>[3x]SLSPAVQTFWKWLQEEGVITAKTPVKASVVTEGLGLVALKDISRNDVILQVPKRLWINPDAVAASEIGRVCSELKPWLSVILFLIRERSREDSVWKHYFGILPQETDSTIYWSEEELQELQGSQLLKTTVSVKEYVKNECLKLEQEIILPNKRLFPDPVTLDDFFWAFGILRSRAFSRLRNENLVVVPMADLINHSAGVTTEDHAYEVKGAAGLFSWDYLFSLKS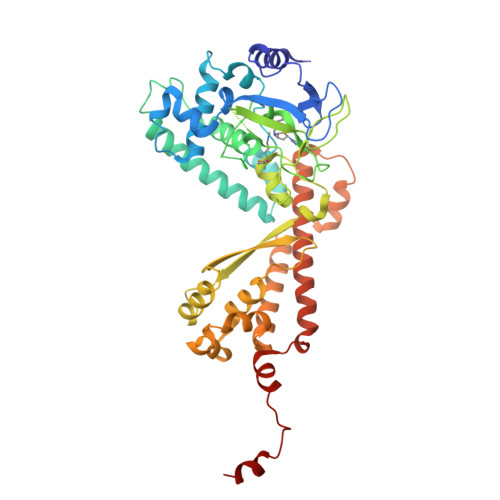PLSVKAGEQVYIQYDLNKSNAELALDYGFIEPNENRHAYTLTLEISESDPFFDDKLDVAESNGFAQTAYFDIFYNRTLPPGLLPYLRLVALGGTDAFLLESLFRDTIWGHLELSVSRDNEELLCKAVREACKSALAGYHTTIEQDRELKEGNLDSRLAIAVGIREGEKMVLQQIDGIFEQKELELDQLEYYQERRLKDLGLCGENGDILENLYFQ>[2x]MTVSASKTAQQLKYIKDSIKTIPDYPKAGILFRDVTSLLENPKAYSASIELLSEHYSESGVTKVVGTEARGFLFGA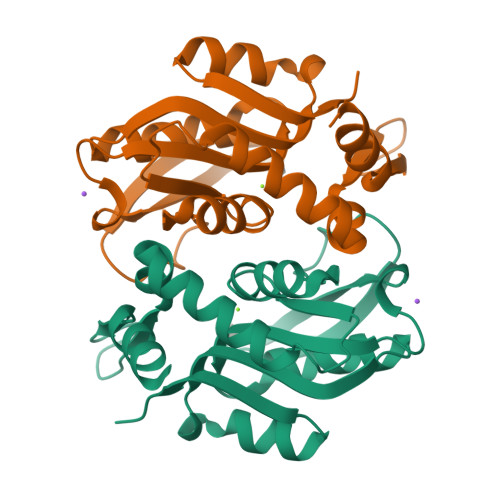PVALALGVGFVPVRKPGKLPRETISESYELEYGTDTLEIHTDSIQPGDKVLVVDDLLATGGTIEATVKLIRRLGGEVVHAAFIINLPELGGEARLTQQGIHCYSLVSFDGH> SFFYDRSTLSSVLQSTSDVSSKFTPSTAKNLQNSILLTPLPSDIVNNSVLPEQERWISFASPTTQKPPYKTKQDWNFIMFSPFTYYKCDLEVTLSKNDRETISSVVRYVPCGAPSDLSDQTMPQTPSLADTRDPHMWVVGQGTTNQISFVIPYTSPLSVLPSV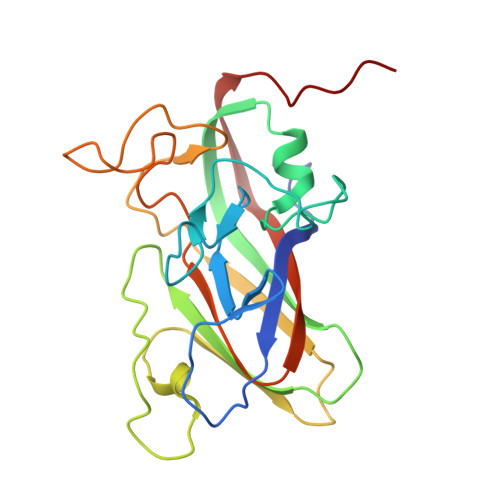WFNGFSNFDNSSRFGVAPNADFGRLLLQGQGTFSVHYRYKKMRVFCPRPTVFIPWP Gelsolin is the prototype of a large superfamily of proteins, responsible for the assembly, disassembly and scavenging of actin filaments by means of its severing and capping activities. Gelsolin is organized into six homologous domains (G1–G6), sharing the same gelsolin-like fold. Each of these modules hosts at least one calcium-binding site and the presence of calcium induces both subtle local and large global conformational changes. Conversely, the presence of mutations in plasma gelsolin is known to be directly related to a rare form of amyloidosis, hereafter referred as AGel amyloidosis (AGel, OMIM reference number 105120).

Here, we report the crystal structure of the second domain of gelsolin carrying the recently identified Gly167Arg mutation. Contrary to the previously published gelsolin G2 crystal structures, two molecules were present in the asymmetric unit and during refinement we observed a discontinuity in the electron density corresponding to a loop connecting β-strand β1 to β2 (hereafter named as the hinge loop). Indeed, such discontinuity was owing to an unusual conformation of the crystallographic dimer, with the N-terminal β1 strand of each monomer contributed from the other polypeptide chain. The dimerization interface between the two monomers mainly involves the swapped β1 strand, comprising residues 158–166, covering a total contact area of 2375 Å2. In addition, the two stretched hinge loops interact in a pseudo β-antiparallel fashion, contributing several polar interactions to the assembly. Contrary to this, the stretched conformation of the hinge loop adopted in the Gly167Arg dimer better accommodates the bulky residue, eliminating the torsional strain. Therefore, the Gly167Arg mutant triggers the conformational change to release both the torsional strain and the repulsion among the basic residues. Similarly, in the Gly167Arg dimer structure, we could only model up to residue 257 and 258 in chains A and B, respectively. In the other G2 structures, calcium is hexacoordinated by Gly186, Asp187, Glu209 and Asp259, but the last residue is disordered in the Gly167Arg mutant and, in its place, we observed a citrate molecule in both subunits. Citrate was derived from the crystallization condition (0.1 M concentration) and was H-bonded to residues 186, 204, 206 and the mutated 167 residue.

>[2x]GSHHVVPNEVVVQRLFQVKRRRVVRATEVPVSWESFNNGDCFILDLGNNIHQWCGSNSNRYERLKATQVSKGIRDNERSGRARVHVSEEGTEPEAMLQVLGPKPALPAGTEDTAKEDAA>[4x]MGSSHHHHHHSSGENLYFQSHMSAPTMSTHLADHYNQAWLFAARAHRNQTLSGSPLPYLVHLGMVA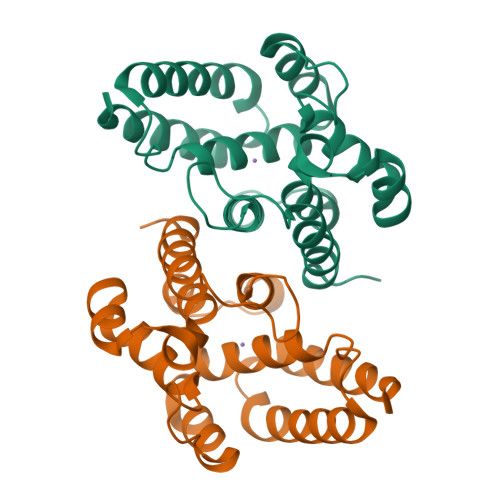NELLAADRDGAIERLGETLQIAVLHDTLQDTATSPEELRQQFGEFVCAGVQALSKRVGDGPKRSLDDYLQALAEGPAQYALVKLCDRITNLQPPPQTWNQDKIANYHQESQLILARLGHAHAATARRLREKIEHYRQYY> LEADKCKEREEKIILVSSANEIDVRPCPLNPNEHKGTITWYKDDSKTPVSTEQASRIHQHKEKLWFVPAKVEDSGHYYCVVRNSSYCLRIKISAKFVENEPNLCYNAQAIFKQKLPVAGDGGLVCPYMEFFKNENNELPKLQWYKDCKPLLLD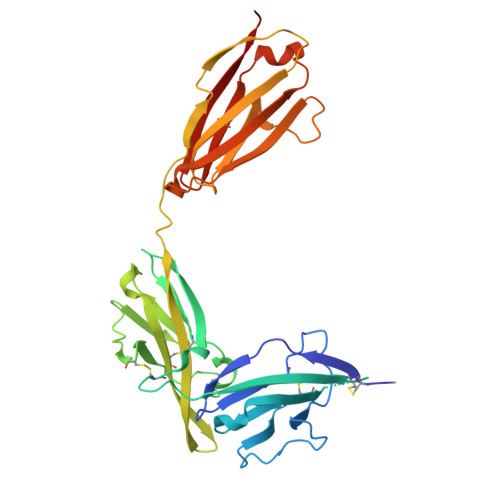NIHFSGVKDRLIVMNVAEKHRGNYTCHASYTYLGKQYPITRVIEFITLEENKPTRPVIVSPANETMEVDLGSQIQLICNVTGQLSDIAYWKWNGSVIDEDDPVLGEDYYSVENPANKRRSTLITVLNISEIESRFYKHPFTCFAKNTHGIDAAYIQLIYPVTNFQK> RSMETGEVVDCHLSDMLQQLHSVNASKPSERGLVRQEEAEDPACIPIFWVSKWVDYSDKYGLGYQLCDNSVGVLFNDSTRLILYNDGDSLQYIERDGTESYLTVSSHPNSLMKKITLLKYFRNYMSEHLLKAGANITPREGDELARLPYLRTWFRTRSAIILHLSNGSVQINFFQDHTKLILC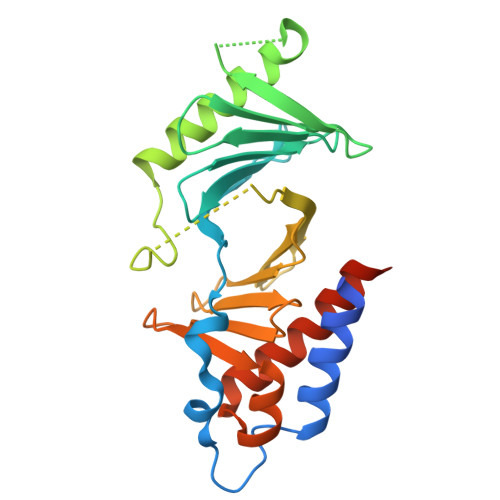PLMAAVTYIDEKRDFRTYRLSLLEEYGCCKELASRLRYARTMVDKLLSSRSASNRLKAS>MDSSRTIGLYFDSALPSSNLLAFPIVLQDIGDGKKQIAPQYRIQRLDSWTDSKEDSVFITTYGFIFQVGNEEVTVGMISDNPKHELLSAAMLCLGSVPNVGDLVELARACLTMVVTCKKSATDTERMVFSVVQAPQVLQSCRVVANKYSSVNAVKHVKAPEKIPGSGTLEYKVNFVSLTVVPRKDVYKIPTAALKVSGSSLYNLALNVTIDVEVDPKSPLVKSLSKSDSGYYANLFLHIGLMSTVDKKGKKVTFDKLERKIRRLDLSVGLSDVLGPSVLVKARGARTRLLAPFFSSSGTACYPISNASPQVAKILWSQTARLRSVKVIIQAGTQRAVAVTADHEVTSTK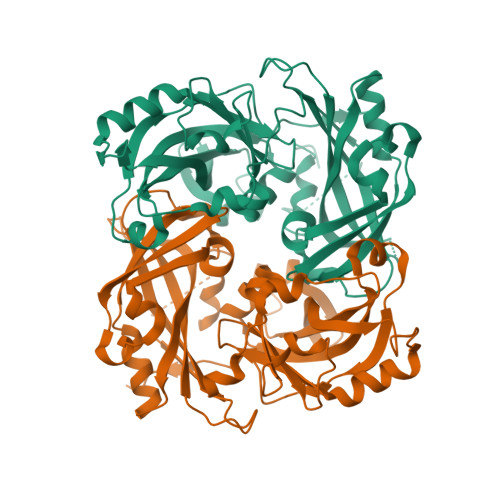IEKRHTIAKYNPFKK[2x]> SNRLDGKVAIITG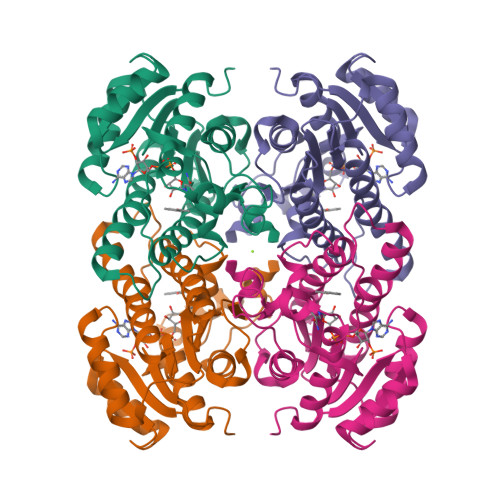GTLGIGLAIATKFVEEGAKVMITGRHSDVGEKAAKSVGTPDQIQFFQHDSSDEDGWTKLFDATEKAFGPVSTLVNNAGIAVNKSVEETTTAEWRKLLAVNLDGVFFGTRLGIQRMKNKGLGASIINMSSIEGFVGDPSLGAYNASKGAVRIMSKSAALDCALKDYDVRVNTVHPGYIKTPLVDDLPGAEEAMSQRTKTPMGHIGEPNDIAYICVYLASNESKFATGSEFVVDGGYTAQ> DYKDDDDKAEVKKIPTMIEGFDDISHGGLPQGATTLVSGTSGTGKTLFAVQFLYNGITIFNEPGIFVTFEESPQDIIKNALSFGWNLQSLIDQGKLFILDASPDPDGQEVAGDFDLSALIERIQYAIRKYKATRVSIDSVTAVFQQYDAASVVRREIFRLAFRLAQLGVTTIMTTERVDEYGPVARFGVEE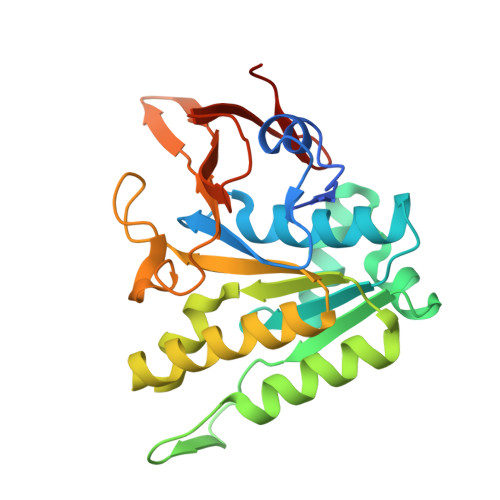FVSDNVVILRNVLEGERRRRTVEILKLRGTTHMKGEYPFTINNGINIFDYKDDDDK>MQTKKNEIWVGIFLLAALLAALFVCLKAANVTSIRTEPTYTLYATFDNIGGLKARSPVSIGGVVVGRVADITLDPKTYLPRVTLEIEQRYNHIPDTSSLSIRTSGLLGEQYLALNVGFEDPELGTAILKDGDTIQDTKSAMVLEDLIGQFLYGSKGDDNKNSGDAPAAAPGNNETTEPVGTTK[6x];>[2x]MSESLSWMQTGDTLALSGELDQDVLLPLWEMREEAVKGITCIDLSRVSRVDTGGLALLLHLIDLAKKQGNNVTLQGVNDKVYTLAKLYNLPADVLPRHHHHHHHH;>MLLNALASLGHKGIKTLRTFGRAGLMLFNALVGKPEFRKHAPLLVRQLYNVGVLSMLIIVVSGVFIGMVLGLQGYLVLTTYSAETSLGMLVALSLLRELGPVVAALLFAGRAGSALTAEIGLMRATEQLSS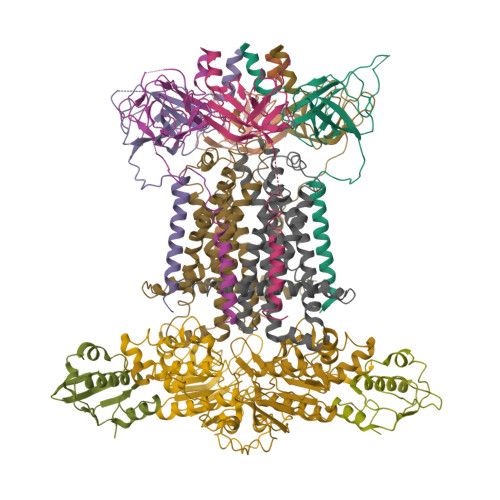MEMMAVDPLRRVISPRFWAGVISLPLLTVIFVAVGIWGGSLVGVSWKGIDSGFFWSAMQNAVDWRMDLVNCLIKSVVFAITVTWISLFNGYDAIPTSAGISRATTRTVVHSSLAVLGLDFVLTALMFGN[2x];>MEQSVANLVDMRDVSFTRGNRCIFDNISLTVPRGKITAIMGPSGIGKTTLLRLIGGQIAPDHGEILFDGENIPAMSRSRLYTVRKRMSMLFQSGALFTDMNVFDNVAYPLREHTQLPAPLLHSTVMMKLEAVGLRGAAKLMPSELSGGMARRAALARAIALEPDLIMFDEPFVGQDPITMGVLVKLISELNSALGVTCVVVSHDVPEVLSIADHAWILADKKIVAHGSAQALQANPDPRVRQFLDGIADGPVPFRYPAGDYHADLLPGS[2x]> MDKYTALIHDENFSTLTLNVSRYPKSLAYWEKLLNYIVKASAPICKSTEPQLLKLIRCTYSSMLNEFPYLENYYIDFALLEYKLGNVSMSHKIFQRGLQAFNQRSLLLWTSYLKFCNNVISHQKQLFKKYETAEEYVGLHFFSGEFWDLYLEQISSRCTSSKKYWNVLRKILEIPLHSFSKFYALWLQRIDDIMDLKQLSQLTSKDELLKKLKIDINYSGRKGPYLQDAKKKLKKITKEMYMVVQYQVLEIYSIFESKIYINYYTSPETLVSSDEIETWIKYLDYTITLQTDSLTH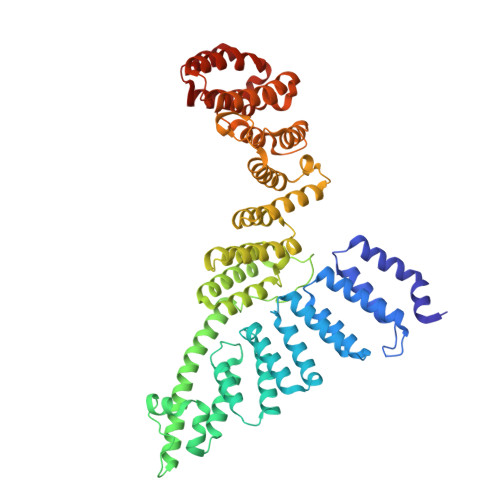LNFQRALLPLAHYDLVWIKYSKWLINSKNDLLGAKNVLLMGLKFSLKKTEIIKLLYSVICKLNEYVLLRNLLEKIESSYSDNVENVDDFEIFWDYLQFKTFCQNSLYSSRYSDSQSNGLLNKELFDKVWKRLSCKEKKSGQEILLNNLVQFYSKDTVEFVEKNIFQKIIEFGWEYYLQNGMFWNCYCRLIYFDTSRSYLDKRQYIVRKIWPQIDKKFAQSVLPSLTEFCESYFPEEMDTLEEMFTEEP>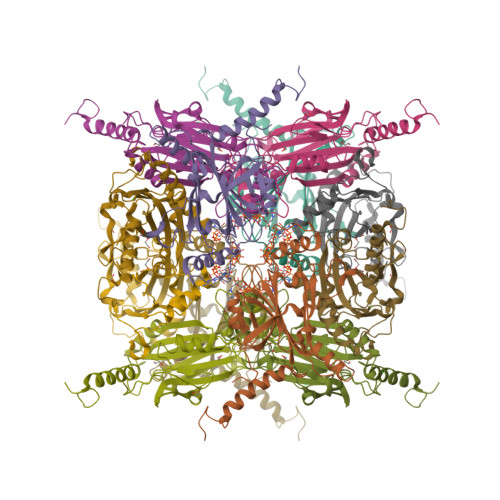 XADVAGTSNRDFKGREQRLFNSEQYNYNNSLNGEVSVWVYAYYSDGSVLVINKNSQYKVGISETFKALKEYREGQHNDSYDEYEVNQSIYYPNGGDARKFHSNAKPRAIQIIFSPSVNVRTIKMAKGNAVSVPDEYLQRSHPWEATGIKYRKIKRDGEIVGYSHYFELPHEYNSISLAVSGVHKNPSSYNVGSAHNVMDVFQSCDLALRFCNRYWAELELVNHYISPNAYPYLDINNHSYGVALSNRQ>MKEEFSYEILEEVAVLSENARGWRKELN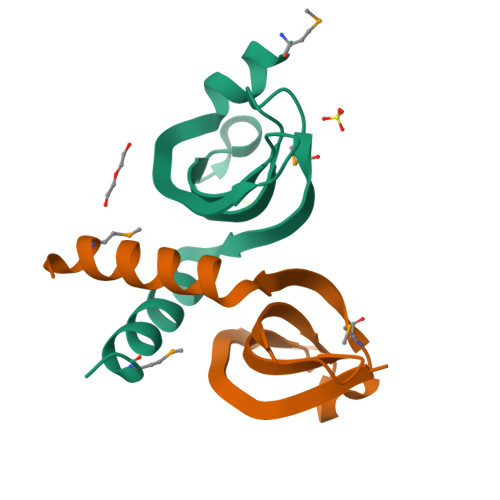LISWNGRPPKFDLREWAPDHEKMGKGITLTNEEFAELSKTIKSMLEHHHHHH[2x]>MNENEPVSIWM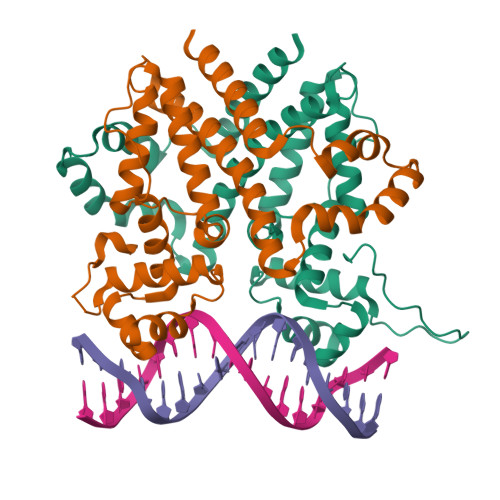HPEPAGRRSARSHRTLSRDQIVRAAVKVADTEGVEAASMRRVAAELGAGTMSLYYYVPTKEDLVELMVDEVIGETRLPDRPGPDWRAALTLAANEKRALWLRHPWLATAWRNGHPVWGPNSLRQQEFVLGTLGVFDLQVDELLSLIGLYNGYVESFVRNEVGWLEEARRTKVDMREWMRRSGPYAQQLVDSGEYPMFARVLAETVAPHMGPDQRFRSGLERLLDSIGASLDRLSPPGRSAASERPALALEHHHHHH[4x]> GSHMGSASEQRVTLTNADKVLYPATGTTKSDIFDYYAGVAEVMLGHIAGRPATRKRWPNGVDQPAFFEKQLALSAPPWLSRATVAHRSGTTTYPIIDSATGLAWIAQQAALEVHVPQWRFVAEPGSGELNPGPATRLVFDLDPGEGVMMAQLAEVARAVRD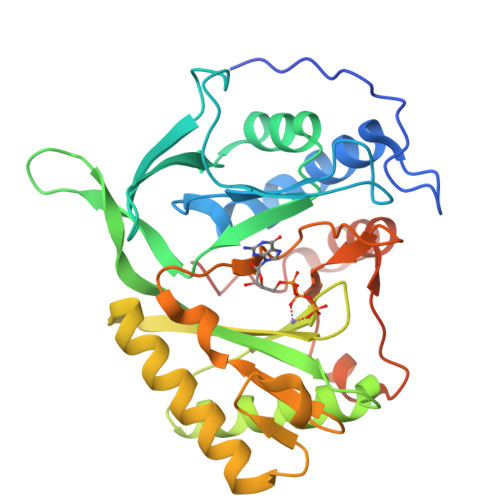LLADIGLVTFPVTSGSKGLHLYTPLDEPVSSRGATVLAKRVAQRLEQAMPALVTSTMTKSLRAGKVFVDWSQNSGSKTTIAPYSLRGRTHPTVAAPRTWAELDDPALRQLSYDEVLTRIARDGDLLERLDADAPVADRLTRY> AKLTIESTPFNVAEGKEVLLLAHNLPQNRIGYSWYKGERVDGNSLIV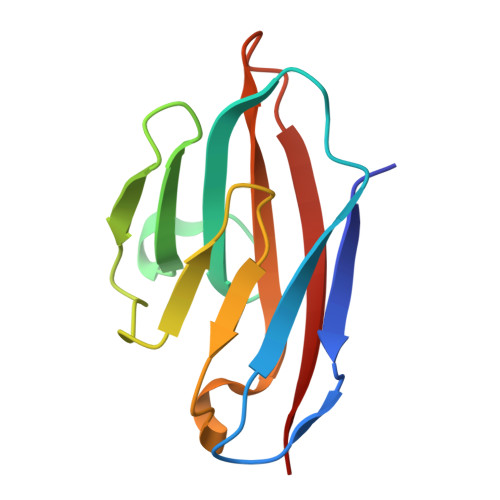GYVIGTQQATPGPAYSGRETIYPNASLLIQNVTQNDTGFYTLQVIKSDLVNEEATGQFHVY> ALLDETPLPPGSRLDVRAYTTVLHALSRAGRYERALELFAELRRQGVAPTVVTYNTLIDGLCKAGKLDEALKLFEEMVEKGIKPDVVTYNTLIDGLCKAGKLDEALKLFEEMVEKGIKPDVVTYNTLIDGLCKAGKLDEALKLFEEMVEKGIKPDVVTYNTLIDGLCKAGKLDEALKLFEEMVEKGIKPDVVTYSTLIDGLCKAGKLDEALKLFEEMVEKGIKPNVVTYSTLIDGLCKAGKLDEALKLFEEMVEKGIKPNVVTYNTLIDGLCKAGKLDEALKLFEEMVEKGIKPDVVTYNTLIDGLCKAGKLDEALKLFEEMVEKGIKPDVVTYNTLIDGLCKAGKLDEALKLFEEMVEKGIKPDVVTYNTLIDGLCKAGKLDEALKLFEEMVEKGIKPDELTYRRVVESYCRAKRFEEARGFLSEV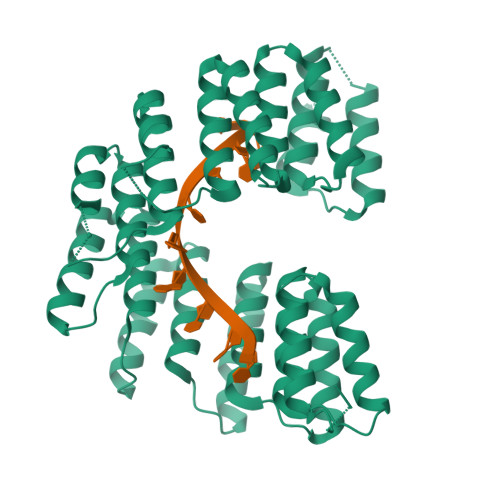SETDLDFDKKALEAYIEDAQFGRLEHHHHHHHH> GSFDLDDVQPNKAVEPEKTKVNYTDEETQKRKKEELDKLMEPALGYVTKIPVNIPSVRKTEISEIDTVTDESLSLVPNEDKLRTIANENYGSVVTKSGSNTMNFVRSGYTIDVVHYGLRDKGYVYYKGVHPSKELPKGNIIVYQGEWDFTSNADLDAKRPNYNPEFNGYGAGQEVGVTSADAKERTYISKFNIDFSNKKLNGQLLTKTKENQEKLRYTVEANISGNRFRGKATATDKTDPILGKDSEHLEGGLYGPKSEELAGKFVAHDKSLFAVFSGKRGNDVLETVKIIDASKIDLTTFESSELNNFGNANVLIIDGQKIDLAGADFKNRKTVDINGKTMVAIACCSNLEYMKFGQLWQKEGEQTKDNSLFLQGERTATDKIPVGGNYKYVGTWDALVSKGTNWVAEADNNRE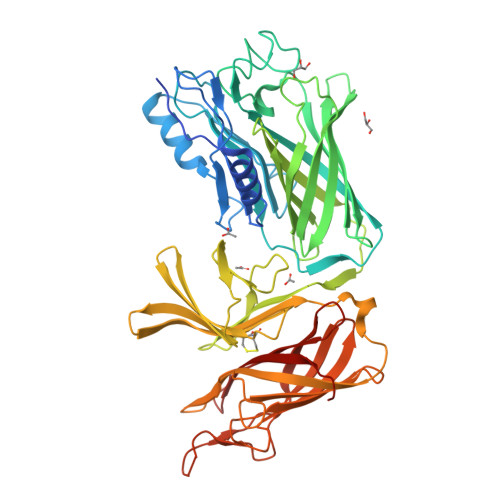SGYRSEFDVNFGDKKVSGKLFDKGGIVPVFMINADIKGNGFTGTANTTDTGFALDSGSSQHGNAVFSDIKVNGGFYGPTAGELGGQFHHKSDNGSVGAVFGAKRQIEK> MAQKLWGSCLFSLFMAALAQETLNPQKSKVDCNKGVTGTVYEYGANTIDGGEFVNFQQYAGKHILFVNVASFCGLTAT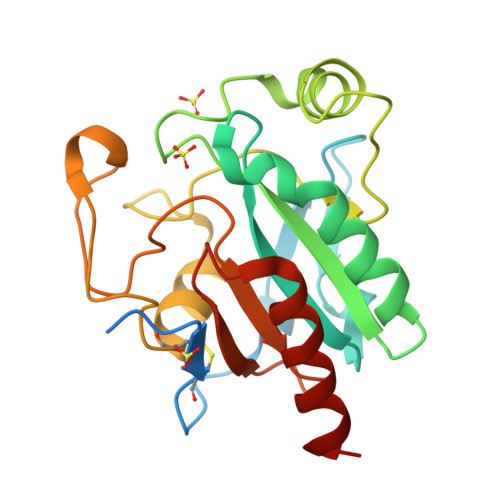YPELNTLQEELKPFNVTVLGFPCNQFGKQEPGKNSEILLGLKYVRPGGGYVPNFQLFEKGDVNGDNEQKVFSFLKNSCPPTSELFGSPEHLFWDPMKVHDIRWNFEKFLVGPDGVPVMRWFHHTPVRIVQSDIMEYLNQTSTQ>[2x]MNYARFITAASAARNPSPIRTMTDILSRGPKSMISLAGGLPNPNMFPFKTAVITVENGKTIQFGEEMMKRALQYSPSAGIPELLSWLKQLQIKLHNPPTIHYPPSQGQMDLCVTSGSQQGLCKVFE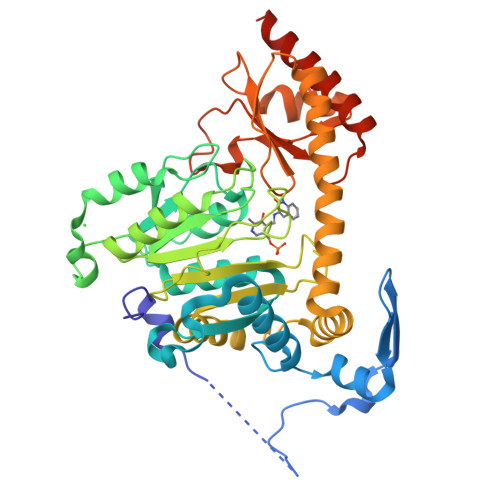MIINPGDNVLLDEPAYSGTLQSLHPLGCNIINVASDESGIVPDSLRDILSRWKPEDAKNPQKNTPKFLYTVPNGNNPTGNSLTSERKKEIYELARKYDFLIIEDDPYYFLQFNKFRVPTFLSMDVDGRVIRADSFSKIISSGLRIGFLTGPKPLIERVILHIQVSTLHPSTFNQLMISQLLHEWGEEGFMAHVDRVIDFYSNQKDAILAAADKWLTGLAEWHVPAAGMFLWIKVKGINDVKELIEEKAVKMGVLMLPGNAFYVDSSAPSPYLRASFSSASPEQMDVAFQVLAQLIKESLLVPRGSLEHHHHHH>GSPAFESYESMELACPAERSGHVAVSDGRH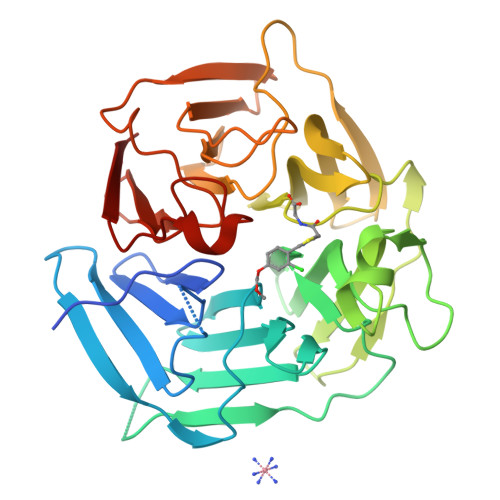MFVWGGYKSNQVRGLYDFYLPREELWIYNMETGRWKKINTEGDVPPSMSGSCAVCVDRVLYLFGGHHSRGNTNKFYMLDSRSTDRVLQWERIDCQGIPPSSKDKLGVWVYKNKLIFFGGYGYLPEDKVLGTFEFDETSFWNSSHPRGWNDHVHILDTETFTWSQPITTGKAPSPRAAHACATVGNRGFVFGGRYRDARMNDLHYLNLDTWEWNELIPQGICPVGRSWHSLTPVSSDHLFLFGGFTTDKQPLSDAWTYCISKNEWIQFNHPYTEKPRLWHTACASDEGEVIVFGGCANNLLVHHRAAHSNEILIFSVQP[2x]>[2x]GPGMTIKGSGSAAFEGTRLCPRVIKPDGPATILAIGTSN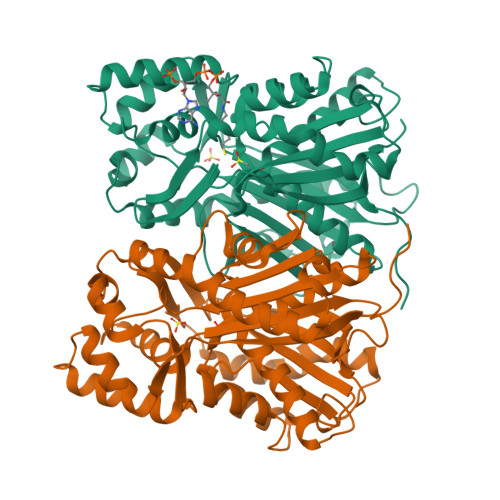PTNIFEQSTYPDFFFDVTNCNDKTELKKKFQRICDKSGIKKRHFHLTDEILRKNPSICKFKEASLDPRQDIAVLEVPKLAKEAAISAIKQWGQPKSKITHLVFATTSGVDMPGADFQLAKLLGLRPTVKRVMLYQQGCYAGATVLRVAKDLAENNKGARVLVACSEVTAVTFRAPSETHLDGLVGSALFGDGAAALIVGSDPVPQEEKPLFEIHWAGEAVLPDSDGAINGHLREAGLIFHLLKDVPGLISKNIDKVLAEPLEYVHFPSYNDMFWAVHPGGPAILDQIEAKLGLSTDKMQASRDVLASYGNMSSASVLFVLDQIRKNSEELHLPTTGEGFEWGFVIGFGPGLTVETLLLRSINI> GQPRVISTIQTGATWEPLGREEPLTVPEVHFRVKHSPFKSELVRYGQFQFNDAAWSLQGSYSCASCHYERGQTTGLIWDLGDEGWGSWKNTKYIRGGRYLPPFRHEGFTGHPDEIVGATS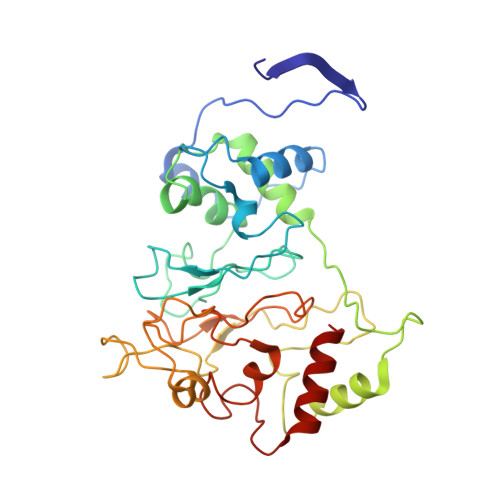SLDRVCGRDPGFVFRSENFSPMRLEALICYIRALEFTGSPFRNADGSLTEAQKRGQKIFEDPKVGCLECHPGDPMDPRALFSDAQTHDVGTGRVGVNGFRSTPGKVFNISALEAGEDPYGVESNTPIIGLDLVKEFDTPTLRDIYASGTYFHDGGARTLMDTINNTVNDKDMHGRTSHLKQQELQDLVEYLKAL> G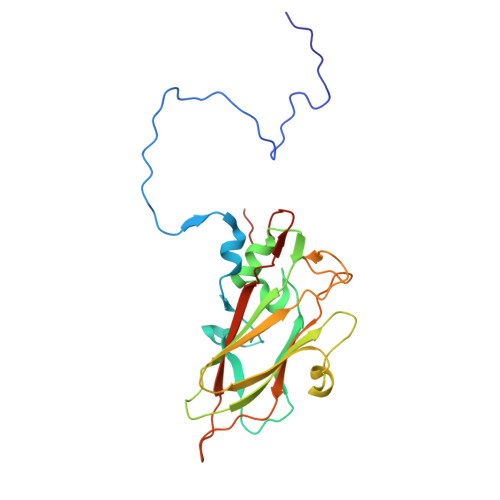LPTVLTPGSEQFLTTDDRQSPSAMPNYEPTPLIHIPGEVKNLLEIAQVDTLIPLNNTTNTTGLGMYRIPLVQNMQGEQVFGFRLYLGDGVLKTTLLGELCQYFTHWAGSLRLSFMYTGPALSSAKLLIAYTPPGAQGPTKRKEAMLGTHVVWDIGLQSTVVLNIPWTSGVQYRYTDPDTYTSAGFVSCWYQTSLVLPPQTQQTVYMLGFISACPDFKLRLMKDTQSIHQE> QVRPFLEVHERSACQARETLVPILQEYPDEISDIFRPSCVAVL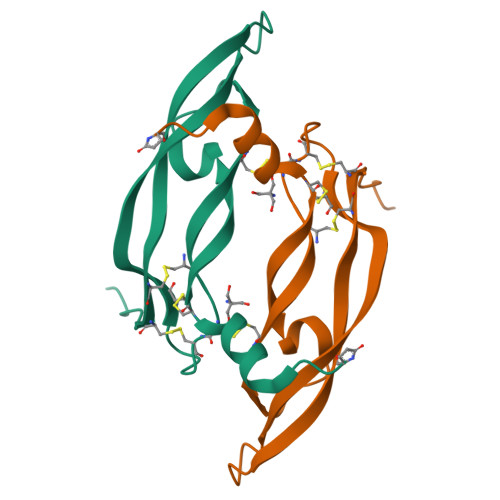RCSGCCTDESLKCTPVGKHTVDIQIMRVNPRTQSSKMEVMKFTEHTACECRPRRKQGEPDGPKEKPR>[2x]GPGSDNKEQTTDQPLAKDKVALLIGNMNYREHPKLKAPLVDVYELTNLLRQLDFKVVSLLDLTEYEMRNAVDEFLLLL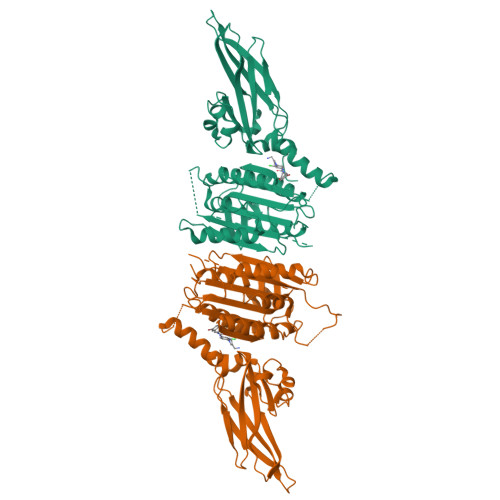DKGVYGLLYYAGHGYENFGNSFMVPVDAPNPYRSENCLCVQNILKLMQEKETGLNVFLLDMCRKRNDYDDTIPILDALKVTANIVFGYATCQGAEAFEIQHSGLANGIFMKFLKDRLLEDKKITVLLDEVAEDMGKCHLTKGKQALEIRSSLSEKRALTDPIQGTEYSAESLVRNLQWAKAHELPESMCLKFDCGVQIQLGFAAEFSNVMIIYTSIVYKPPEIIMCDAYVTDFPLDLDIDPKDANKGTPEETGSYLVSKDLPKHCLYTRLSSLQKLKEHLVFTVCLSYQYSGLEDTVEDKQEVNVGKPLIAKLDMHRGLGRKTCFQ> GGUGGGGACGA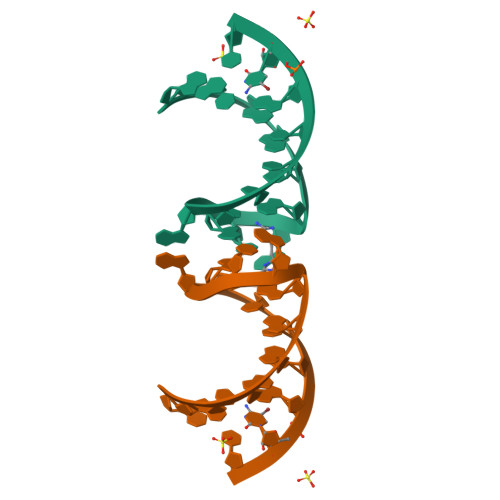CCCCACC>[2x]RSENITQWNLQDNGTEGIQRAMFQRGVNRSLKGI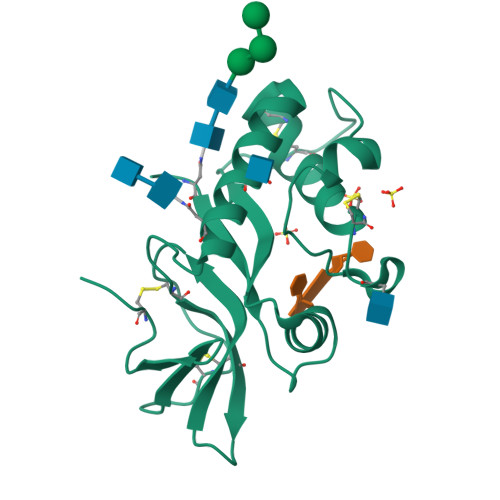WPEKICTGVPSHLATDTELKAIHGMMDASEKTNYTCCRLQRHEWNKHGWCNWYNIEPWILLMNKTQANLTEGQPLRECAVTCRYDRDSDLNVVTQARDSPTPLTGCKKGKNFSFAGILVQGPCNFEIAVSDVL(2~{R},4~{S},5~{S},6~{S})-5-acetamido-4-oxidanyl-6-[(1~{R},2~{R})-1,2,3-tris(oxidanyl)propyl]-2-[[(2~{R},3~{R},4~{S},5~{R},6~{S})-3,4,5-tris(oxidanyl)-6-[(2~{R},3~{S},4~{R},5~{R})-1,2,4,5-tetrakis(oxidanyl)-6-oxidanylidene-hexan-3-yl]oxy-oxan-2-yl]methoxy]oxane-2-carboxylic acid | C23 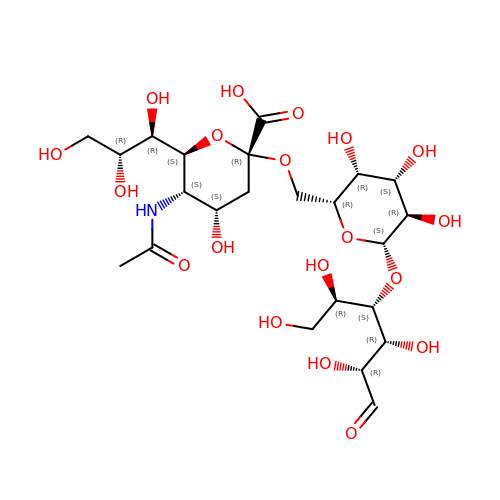H39 N O19 | VMWYCXKMRSTDSP-DKHYMJAUSA-N> GPLGSPEFIILQTYRAIADYEKTSGSEMALSTGDVVEVVEKSESGWWFCQMKAKRGWIPASFLEPLDSPDETEDPEPNYAGEPYVAIKAYTAVEGDEVSLLEGEAVEVIHKLLDGWWVIRKDDVTGYFPSMYLQKSGQDVSQAQRQIKRGAPPRRSSIRNAHSIHQRSRKRLSQDAYRRNSVRFLQ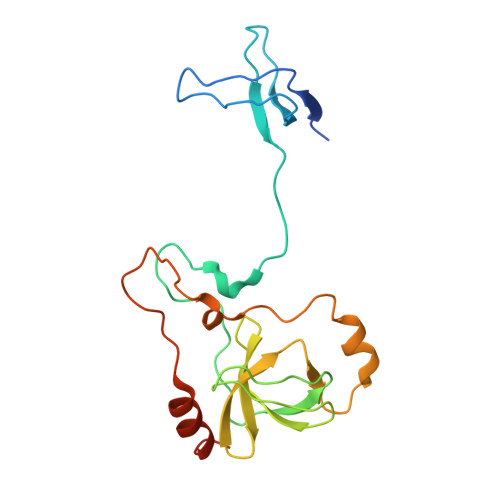QRRRQAR>MTTKQICFADRCFNFAFGEHVLESVESYIPRDEFDQYIMISDSGVPDSIVHYAAEYFGKLAPVHILRFQGGEEYKTLSTVTNLQERAIALGANRRTAIVAVGGGLTGNVA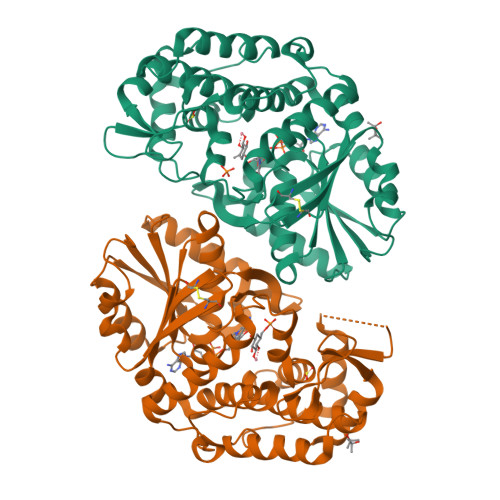GVAAGMMFRGIALIHVPTTFLAASDSVLSIKQAVNLTSGKNLVGFYYPPRFVFADTRILSESPPRQVKAGMCELVKNMLILENDNKEFTEDDLNSANVYSPKQLETFINFCISAKMSVLSEDIYEKKKGLIFEYGHTIGHAIELAEQGGITHGEAIAVGMIYAAKIANRMNLMPEHDVSAHYWLLNKIGALQDIPLKSDPDSIFHYLIHDNKRGYIKLDEDNLGMILLSGVGKPAMYNQTLLTPVRKTLIKEVIREGL[2x]>[2x]MDLVEEILRLKEERNAIILAHNYQLPEVQDIADFIGDSLELARRATRVDA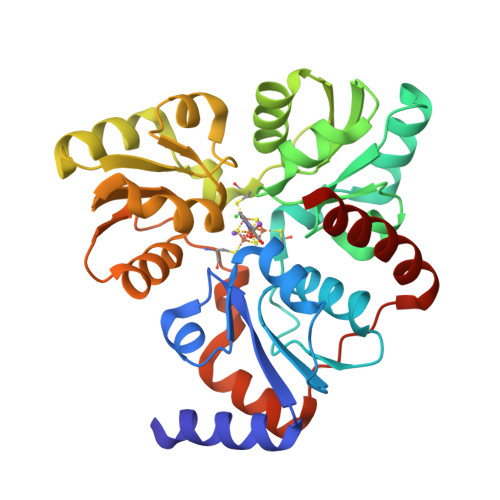DVIVFAGVDFMAETAKILNPDKVVLIPSREATCAMANMLKVEHILEAKRKYPNAPVVLYVNSTAEAKAYADVTVTSANAVEVVKKLDSDVVIFGPDKNLAHYVAKMTGKKIIPVPSKGHCYVHQKFTLDDVERAKKLHPNAKLMIHPECIPEVQEKADIIASTGGMIKRACEWDEWVVFTEREMVYRLRKLYPQKKFYPAREDAFCIGMKAITLKNIYESLKDMKYKVEVPEEIARKARKAIERMLEMSK> MTAPRSWAPTTRARGDTEALCSPEDGWVKVHPTPGTMLFREILHGQLGYTEGQGVYNVVRSSEATTRQLQAAIFHALLNATTYRDLEADWLGHVAARGLQPQRLVRRYRNAREADIAGVAERVFDTWRNTLRTTLLDFAHGLVACFAPGGPSGPSSFPKYIDWLTCLGLVPILRKRQEGGVTQGLRAFLKQHPLTRQLATVAEAAERAGPGFFELALAFDSTRVADYDRVYIYYNHRRGDWLVRDPISGQRGECLVLWPPLWTGDRLVFDSPVQRLFPEIVACHSLREHAHVCRLRNTASVKVLLGRKSDSERGVAGAARVVNKVLGEDDETKAGSAASRLVRLIINMKGMRHVGDINDTVRAYLDEAGGHLIDAPAVDGTLPGFGKGGNSRGSAGQDQGGRAPQLRQAFRTAVVNNINGVLEGYINNLFGTIERLRETNAGLATQLQERDRELRRATAGALERQQRAADLAAESVTGGCGSRPAGADLLRADYDIIDVS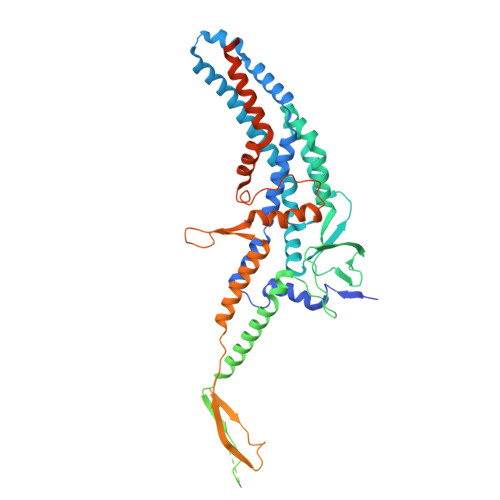KSMDDDTYVANSFQHPYIPSYAQDLERLSRLWEHELVRCFKILCHRNNQGQETSISYSSGAIAAFVAPYFESVLRAPRVGAPITGSDVILGEEELWDAVFKKTRLQTYLTDIAALFVADVQHAALPPPPSPVGADFRPGASPRGRSRSRSPGRTAPGAPDQGGGIGHRDGRRDGRR> SGSFELSVQDLNDLLSDGSGCYSLPSQPCNEVTPRI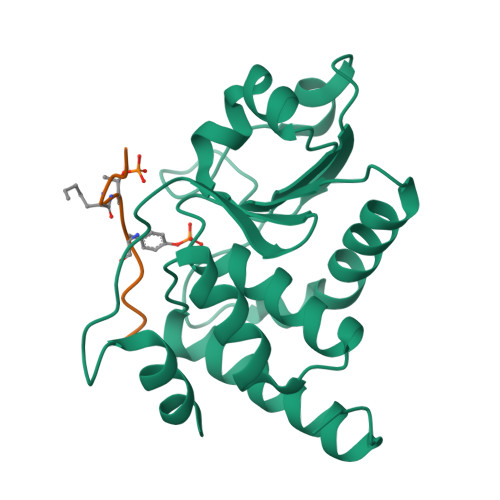YVGNASVAQDIPKLQKLGITHVLNAAEGRSFMHVNTNANFYKDSGITYLGIKANDTQEFNLSAYFERAADFIDQALAQKNGRVLVHSREGYSRSPTLVIAYLMMRQKMDVKSALSIVRQNREIGPNDGFLAQLCQLNDRLAKEGKLKP;> DDEATGYVATR>[3x]XPPGPPGFPGDRGLPGPVGPPGP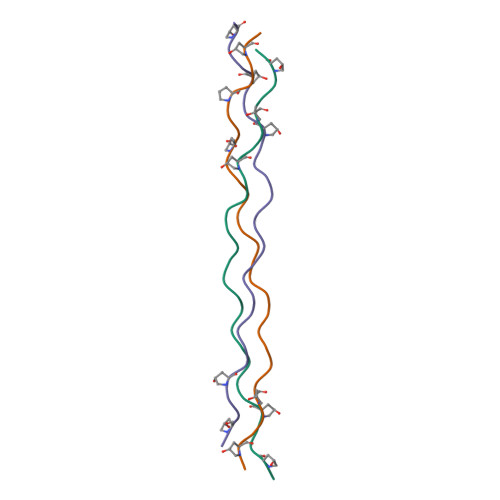PGPPGX>[2x]MKYAGILAGGIGSRMGNVPLPKQFLDLDNKPILIHTLEKFILINDFEKIIIATPQQWMTHTKDTLRKFKISDERIEVIQGGSDRNDTIMNIVKHIESTNGINDDDVIVTHDAVRPFLTHRIIKENIQAALEYGAVDTVIDAI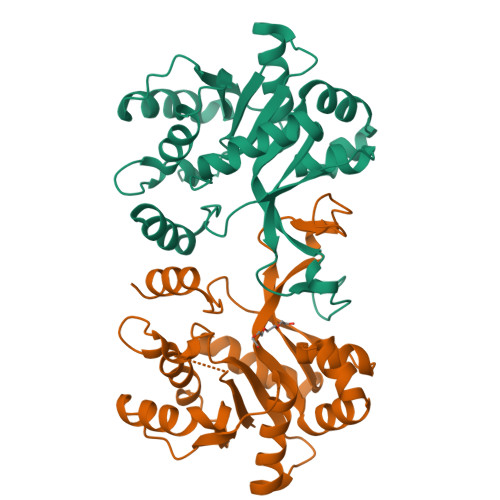DTIVTSKDNQTIDAIPVRNEMYQGQTPQSFNINLLKESYAQLSDEQKSILSDACKIIVETNKPVRLVKGELYNIKVTTPYDLKVANAIIRGGIADDGGSLVPRGSAAAALEHHHHHHHH> MDLSTNLNTGLLPRVNGTPPPEVPLADIELGSLEFWGRDDDFRDGAFATLRREAPISFWPPIELAGLTAGKGHWALTKHDDIHFASRHPEIFHSSPNIVIHDQTPELAEYFGSMIVLDDPRHQRLRSIVSRAFTPKVVARIEASVRERAHRLVAAMIENHPDGQADLVSELAGPLPLQIICDMMGIPEEDHEQIFHWTNVILGFGDPDLTTDFDEFLQVSMAIGGYA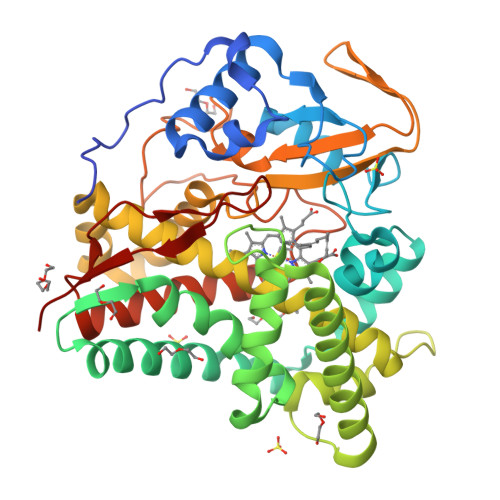TALADDRRVNHHGDLTTSLVEAEVDGERLSSSEIAMFFILLVVAGNETTRNAISHGMLALSRYPDERAKWWSDFDGLAATAVEEIVRWASPVVYMRRTLSQDVDLRGTKMAAGDKVTLWYCSANRDEEKFADPWTFDVTRNPNPQVGFGGGGAHFCLGANLARREIRVVFDELRRQMPDVVATEEPARLLSQFIHGIKRLPVAWSR> MGSSFEVIARTAYEEGRTRLATELLNHEPRAGRQVPLLLSMEEDELALDKAIESGDTDLIYFVIHQLRRKLPLASFFRVVSSRPTASAMVEALARNSDGDGNEDTALLKDLYYQDDRRLDGASVFIREALQQPETRTASDKLDLAANLLQGNQKEHVFELGALKEAKMLLRMQET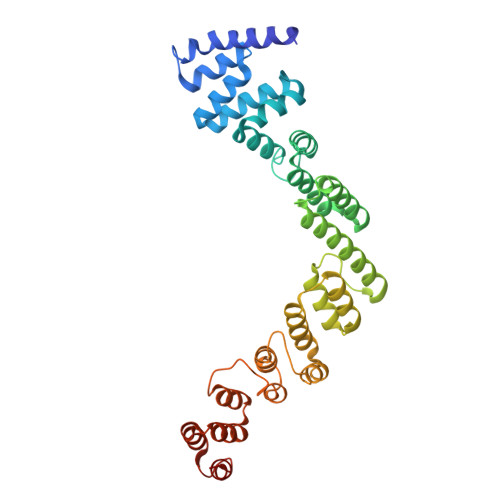FERDLTDSFVGLSVNQTMFKLIKLGYHGRAKKIQSEFKVPERVAWWIRLQALVAKRDWNEIEEISRQRKSPIGWEPFFNQVLQAGNPRLAATFIPKCTNLEPGQTITMYEKCGMRVKAAEEAVRLKDTEAWNRLLEAAGRNTAEGREIERLGATVFKK[2-(pentylamino)ethane-1,1-diyl]bis(phosphonic acid) | C7 H19 N O6 P2 | 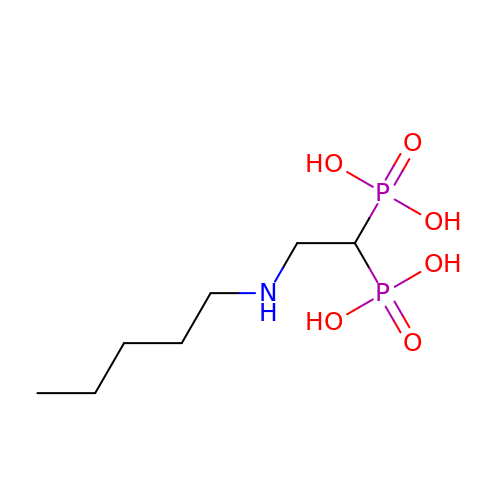YDYMUJPNPOBLGS-UHFFFAOYSA-N TIGECYCLINE 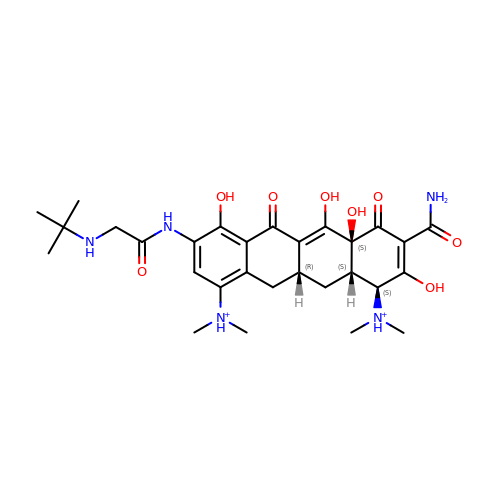| C29 H41 N5 O8 | FPZLLRFZJZRHSY-HJYUBDRYSA-P>TTILSVRKGDTVVLLGDRQVTLGERIVAKSSACKLRRINDDVVIGFAGSTADAISLMEKLENKIGEFPNQLTRAAVELAKEWRTDRALRRLEASLIVCSAEETLEIDGQGNVI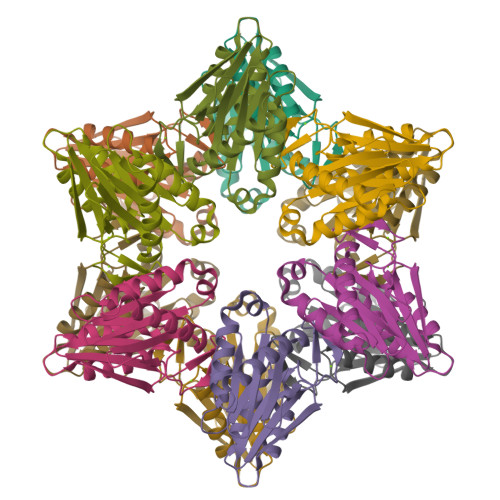TPEADGIVAIGSGGTFAKAAARALIDVDGYDAEKIARKAMRIATDIDVFSNEHWDVEVLEHHHHHH[3x]>SEKETKAFNLKTAKGEEKIDIPKDPKRIVVMAPTYAGGLKYLDANIVGVSDQVD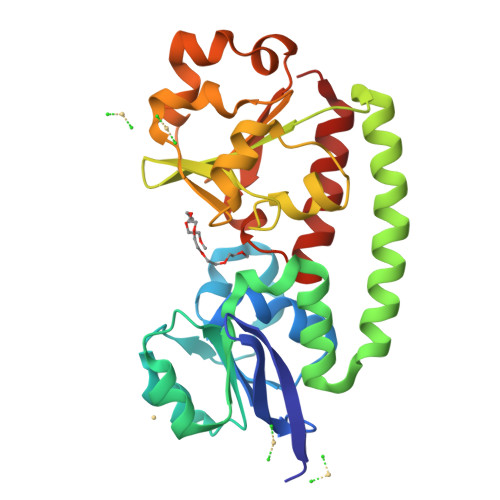QSPVLAKQFKDVDKVGAEDVEKVASLKPDLIITYNTDKNTDKLKKIAPTIAFDYAKYNYLEQQEAMGDIVGKSDEVKKWKADWEKQTAQDSKDIKAHLGDDTSVTIFEDFDKKIYAYGKNWGRGSEVLYQAFGLQMPKALDDATKKEGWTEVPKEEVGKYAGDVIITAKAKDAAQPEFQKTAMWQNLEAVQNKYAFNVDSSVYWYNDPYTLDVIRKDLKKQLLALPTN[2x]>MSLLKIYWRAMQYLAVERTATITMCVASVLVALVTLAEPVLFGRVIQSISDKGDIFSPLLMWAALGGFNIMAAVFVARGADRLAHRRRLGVMIDSYERLITMPLAWHQKRGTSNALHTLIRATDSLFTLWLEFMRQHLTTVVALATLIPVAMTMDMRMSLVLIVLGVIYVMIGQLVMRKTKDGQAAVEKHHHKLFEHVSDTISNVSVVQSYNRIASETQALRDYAKNLENAQFPVLNWWALASGLNRMASTFSMVVVLVLGAYFVTKGQMRVGDVIAFIGFAQLMIGRLDQISAFINQTVTARAKLEEFFQMEDATADRQEPENVADLNDVKGDIVFDNVTYEFPNSGQGVYDVSFEVKPGQTVAIVGPTGAGKTTLINLLQRVFDPAAGRIMIDGTDTRTVSRRSLRHAIATVFQDAGLFNRSVEDNIRVGRANATHEEVHAAAKAAAAHDFILAKSEGYDTFVGERGSQL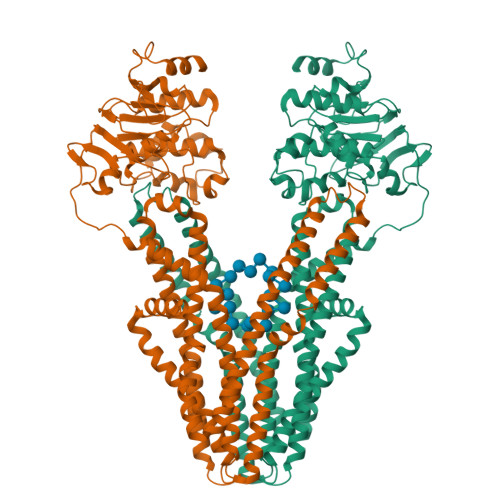SGGERQRLAIARAILKDSPILVLDEATSALDVETEEKVTQAVDELSHNRTTFIIAHRLSTVRSADLVLFMDKGHLVESGSFNELAERGGRFSDLLRAGGLKLEDKQPKQPVVEGSNVMPFPVKGAVA[2x]>GSTGLIKHTEYMEFLKSVPTFQSL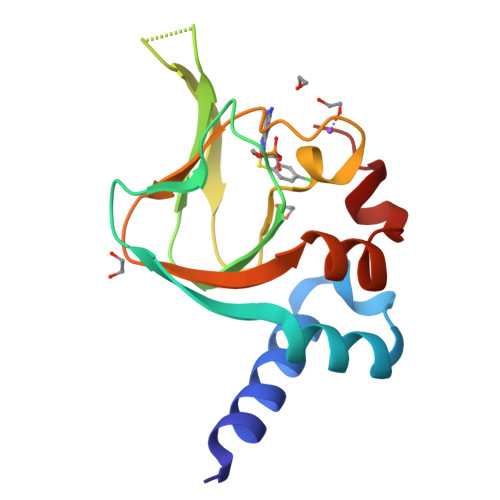PEEILSKLADVLEETHYENGEYIIRQGARGDTFFIISKGTVNVTREDSPSEDPVFLRTLGKGDWFGEKALQGEDVRTANVIAAEAVTCLVIDRDSFKHLIGGLDDVSNKAY[2x]> NFNLEHPFFFTNNDYSTDTSIKYQASLPFNWHEVMNNDEWVYQYPIGKFVERQGWKIHISSEYNSSHELLQDVAKICHEMRIPFKHLSTEDKFIMRNGKLVSRGFSGKFITCYPNQNELESVLQRLESALKQYNGPYILSDKRWDEAPIYLRYGVFRPSRDDEKKVAIDELIVGDEVVKDERLPVFKIPKGIVPPDFLNKWLDKKDKKQGDFPFIIDNAIRFSNSGGIYNARLKEDGKKIILKEARPYTGLGFDGTYSSEKLASECKALKILNEWSEAPKIYWHGKIWEHTFLGIEHMKGVPLNRWVTNNFPLYEVVDKTKDYLLRVSKIVEKLIDLTNKFHSENVYHQDLHLGNILVKDEDEISIIDWEQAVFSNDEKVVHKVAAPGFRAWRETLPSEIDWYGIRQIAHYLYMPLVTTSDLTYNYVSQTRIEGKKLFESLGYTREHIDYVESLLSYLDSKCPQIENISRKKVLKPMHEIRTIESEQDIQDFIIKLLRGFTLTYGQWRKEFQSRFFPVAYYGLNFNQGIAFSDLAILWSYQQLAKKVKNFKFDDYYEIRTQVINEAVNNFKKSSLSGLFDGKIGTIWLIYEFGEIDRAVELFTTHFIEIFENSQNKNLYSGQAGILLVGLYFLSKGEIDNKLGEEILIRLREYTLNYIENPETFCKVGASDVQSNDPYENFGGLLYGHAGVAWLFGEAYKLTGESIYKNGLELAVDKELVAYKVDSNNSLQYSQGHRLLPYLATGSAGLLLLINRNKEILSSKYLKYLTSLERATDVVFCVLPGLFNGFCGLEVANNIYSDIDDNFSGQKKLIEQLYRYLCVIEEGFVIAGDNGLKITTDIASGFAGVAIGLVSIMDNKLTILPQI;> FNLEHPFFFTNNDYSTDTSIKYQASLPFNWHEVMNNDEWVYQYPIGKFVERQGWKIHISSEYNSSHELLQDVAKICHEMRIPFKHLSTEDKFIMRNGKVVSRGFSGKFITCYPNQNELESVLQRLESALKQYNGPYILSDKRWDEAPIYLRYGVFRPSRDDEKKVAIDELIVGDEVVKDERLPVFKIPKGIVPPDFLNKWLDKKDKKQGDFPFIIDNAIRFSNSGGIYNARLKEDGKKIILKEARPYTGLGFDGTYSSEKLASECKALKILNEWSEAPKIYWHGKIWEHTFLGIEHMKGVPLNRWVTNNFPLYEVVDKTKDYLLRVSKIVEKLIDLTNKFHSENVYHQDLHLGNILVKDE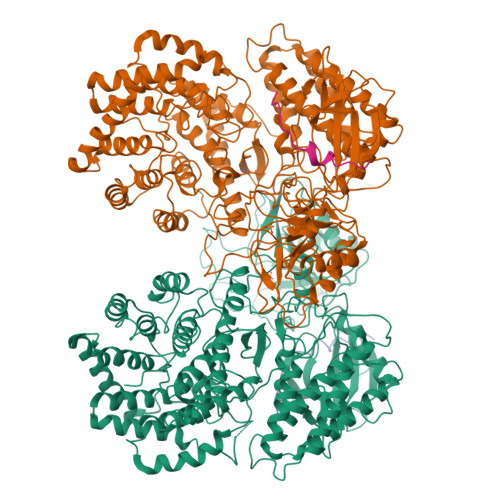DEISIIDWEQAVFSNDEKVVHKVAAPGFRAWRETLPSEIDWYGIRQIAHYLYMPLVTTSDLTYNYVSQTRIEGKKLFESLGYTREHIDYVESLLSYLDSKCPQIENISRKKVLKPMHEIRTIESEQDIQDFIIKLLRGFTLTYGQWRKEFQSRFFPVAYYGLNFNQGIAFSDLAILWSYQQLAKKVKNFKFDDYYEIRTQVINEAVNNFKKSSLSGLFDGKIGTIWLIYEFGEIDRAVELFTTHFIEIFENSQNKNLYSGQAGILLVGLYFLSKGEIDNKLGEEILIRLREYTLNYIENPETFCKVGASDVQSNDPYENFGGLLYGHAGVAWLFGEAYKLTGESIYKNGLELAVDKELVAYKVDSNNSLQYSQGHRLLPYLATGSAGLLLLINRNKEILSSKYLKYLTSLERATDVVFCVLPGLFNGFCGLEVANNIYSDIDDNFSGQKKLIEQLYRYLCVIEEGFVIAGDNGLKITTDIASGFAGVAIGLVSIMDNKLTILPQI;> QGMAEEVLNLQLVSVQVD;> VSMAEEVLNLQLVSVQV>[2x]MAGAIASRMSFSSLKRKQPKTFTVRIVTMDAEMEFNCEMKWKGKDLFDLVCRTLGLRETWFFG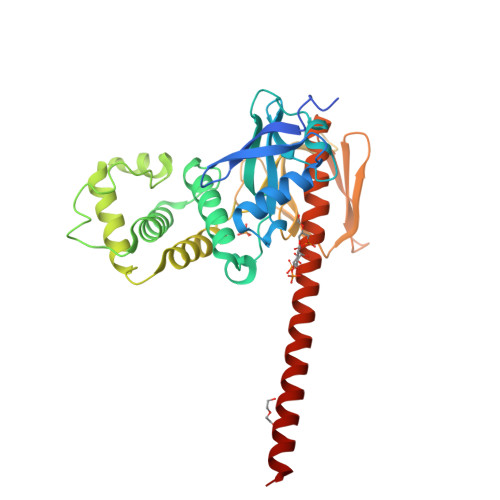LQYTIKDTVAWLKMDKKVLDHDVSKEEPVTFHFLAKFYPENAEEELVQEITQHLFFLQVKKQILDEKIYCPPEASVLLASYAVQAKYGDYDPSVHKRGFLAQEELLPKRVINLYQMTPEMWEERITAWYAEHRGRARDEAEMEYLKIAQDLEMYGVNYFAIRNKKGTELLLGVDALGLHIYDPENRLTPKISFPWNEIRNISYSDKEFTIKPLDKKIDVFKFNSSKLRVNKLILQLCIENHDLFMRRRKADSLEVQQMKAQAREEKARKQMERQRL> MVHYRTIDSPIGPLTLAGHGSVLTNLRMLEQTYEPSRTHWTPDPGAFSGAVDQLNAYFAGELTEFDVELD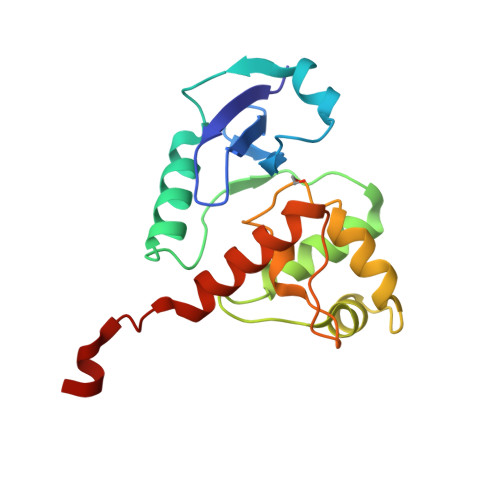LRGTDFQQRVWKALLTIPYGETRSYGEIADQIGAPGAARAVGLANGHNPIAIIVPCHRVIGASGKLTGFGGGINRKRALLELEKSRAPADLTLFD>[5x]MEEKRLSAKKGLPPGTLVYTGKYREDFEIEVMNYSIEEFREFKTTDVESVLPFRDSSTPTWINITGIHRTDVVQRVGEFFGIHPLVLEDILNVHQRPKVEFFENYVFIVLKMFTYDKNLHELESEQVSLILTKNCVLMFQEKIGDVFDPVRERIRYNRGIIRKKRADYLLYSL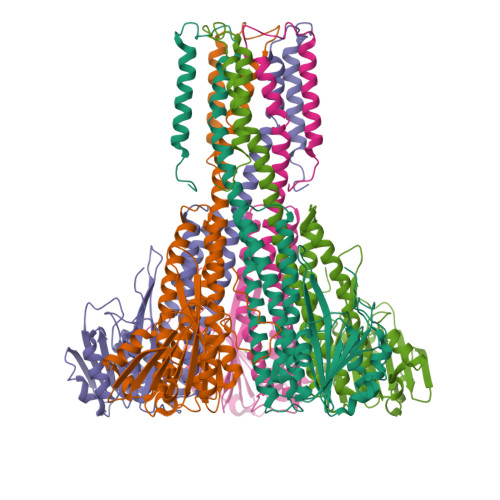IDALVDDYFVLLEKIDDEIDVLEEEVLERPEKETVQRTHQLKRNLVELRKTIWPLREVLSSLYRDVPPLIEKETVPYFRDVYDHTIQIADTVETFRDIVSGLLDVYLSSVSNKTNEVMKVLTIIATIFMPLTFIAGIYGMNFEYMPELRWKWGYPVVLAVMGVIAVIMVVYFKKKKWL Legionella pneumophila is an opportunistic pathogen that causes the potentially fatal pneumonia known as Legionnaires’ disease. The pathology associated with infection depends on bacterial delivery of effector proteins into the host via the membrane spanning Dot/Icm type IV secretion system (T4SS). The Dot/Icm complex of L. pneumophila is one of the largest known T4SSs. The Dot/Icm T4SS has as many as 300 protein substrates, a striking contrast to the H. pylori Cag and B. pertussis Ptl T4SSs, each of which transports only one virulence factor.

(a–b) The outer membrane cap (OMC) disk has been reconstructed to 2.8 Å resolution using C13 symmetry. Models of DotC, DotD1, DotD2, DotH, and DotK were built within the map of the OMC that was reconstructed with C13 symmetry imposed. The asymmetric unit of the OMC is comprised of one copy of DotC (brown), DotF1 (purple), DotK (cyan), DotH (orange), Dis1 (Lpg0657, blue), Dis2 (Lpg0823, green), Dis3 (Lpg2847, tan), and two copies of DotD (red and pink). A DALI search of Dis2 returned no significant structural similarity among PDB entries, making its function difficult to infer. Together, the predicted membrane interaction sites in DotC, DotD1, DotD2, DotK, would anchor the Dot/Icm T4SS to the outer membrane at seven positions per asymmetric unit. Dis2 is positioned near the outer membrane and consists of two lobes, similar in both sequence and structure, that are pinned together with a total of five disulfide bonds, all of which show strong density within the map. We identify ‘chain 2’ as Lpg2847 (residues 29–320), now referred to as Dis3. Dis3, predominantly a β-helical protein, is the major contributor to the ‘arms’ that extend outward radially from the disk of the OMC. Finally, we identified ‘chain 3’ as DotF (DotF1, residues 208–266).

>[13x]MRKFILSLSILLSALLVACSSRNHYGDTGSLAGLQAMADSKYTRAQKKQKMGKIREMALKETALSVGAQAGLAWRAKIIDEQLNKQARNLDAIYDFNSLVLEHNILPPVLLEGRNTLNLADAQSIRISDRTYKVAKQAHFITTPPTWRQYLWMDYVKPEAPNVTLLPKTKAEKEIWCIYTERGWKNGIDQANTILEENIARIKEDFGGMILYRKLLAMNMVSPPYVSHTDLGVTGDGSEIHIDDRVLRITALPELNVNSAEWRAAVAKDENALERFKNMEKLANQAKIVITNKSWQPIIAPVS;>[26x]MNNNKIVIMFIFSALLAGCAGTMKFKKPPINNPSDDATIKLAEAAVSVSDSMLEMAKVEKVITPPSKDNTLTIPNAYNLQARASVDWSGPIEELTARIAKAAHFRFRVLGKSPSVPVLISISTKDESLAEILRDIDYQAGKKASIHVYPNSQVVELRYAKIYS;>MMKKYDQLCKYCLVIGLTFSMSCSIYAADQSDDAQQALQQLRMLQQKLSQNPSPDAQSGAGDGGDNAASDSTQQPNQSGQANAPAANQTATAGGDGQIISQDDAEVIDKKAFKDMTRNLYPLNPEQVVKLKQIYETSEYAKAATPGTPPKPTATSQFVNLSPGSTPPVIRLSQGFVSSLVFLDSTGAPWPIAAYDLGDPSSFNIQWDKTSNTLMIQATKLYNYGNLAVRLRGLNTPVMLTLIPGQKAVDYRVDLRVQGYGPNAKSMPTEEGIPPSANDLLLHVLEGVPPPGSRRLVVSGGDARAWLSNEKMYVRTNLTILSPGWLASMTSADGTHAYEMQKSPVLLVSWHGKVMQLKVEGL[13x];>MRSLRTNYIYVLFKTTGLLFLLLLSACNRSGYIPENEVPKLPCRVDGACDATIIKMMTDLNKKGIKVASVGQNYLISIPASALFADQSPRLNWASYSLLNEIAAFLKQFRKIAITVTSYSSKYVSVKRERALTLARSRVVSEYLWSQGVDSRIIFTQGLGSDKPITSYTLGGDRSPNARVEITFRRAVA[13x];>[13x]MRNLMRCLIMIKSLIKGVDMSRKLAKTRILGYGLMICFLAGCFHPPYNNFQPDRRAVKRVGVDTGIGAVAGAIASGTASGTLIGAAAGGTVGLVASIYRDSKRKIIRDLQKQDIQYVEYGDTRTLIIPTDKYFMFSSPRLNEICYPGLNNVIRLLNFYPQSTIYVAGFTDNVGSRSHKRKLSQAQAETMMTFLWANGIAAKRLKAEGYGDKNAISDNAIIHGSAQNRRIEIQWFTSPAQPPQPQMAYVK;>[13x]MLKRCYLLILLMFVLASCAHHKPQTPPAEVKKQGTSSTRQFRQVSSFNQIVVQGRLNVNLHTGYNKPEVMLRGDPRDLVQVRTIVKQNTLYVSLGQGYPDYGAVTVDIKTKFLNRFRYEGAGVVTGNNLRTSYLDLYLANEGTTRLAGNIGLQKLEAVGNGVTQINGVSSRNLQIVLKGDPKVLISGFVNLRQLDMYGKGTLSLYWIKSDTLTIRAKKAAKIQLAGIVNRLDVELWDFAQFKGKYLRAQRSFVKTHDKSVAEISAVNHQSSLATDASDIYYYNLSKTRADFMAFNGSVLDMREWGQSDLKDFDRYNKQFP;>[13x]MLFLKIKTNQRTTMNILKPKAFLLASVFVLSISPAFAADGCCSKMGGINYCDSSAGRLVCNNGFYSTCYCTRHAVMDLQFLMGCCLWHGGVYPQLNSSGLVVCNDGYVSEECSLQKPVEQISVY;>MMAEHDQNNDEYKFAELDSYDMDQAGESDLDSEASYQSGKEGLTKKKDIKRNALIAIGAVVFIMVMYKIIGWMFFSDKSSQVTSKPAIPPVTQVATPQPVQTIPTTTPIQQVQPTTIIEDDPDLKKKVSAIEMTQQSLRSEVNALSEQINAVNNNIKNLNAQIVNLNQIIGNMSNQIARQSEVINVLMARTTPKKVVKVSRPIVQARIIYYIQAVIPGRAWLIGSNGSTLTVREGSKIPGYGMVKLIDSLQGRILTSSGQVIKFSQEDS[13x]5-O-phosphono-beta-D-ribofuranosylamine 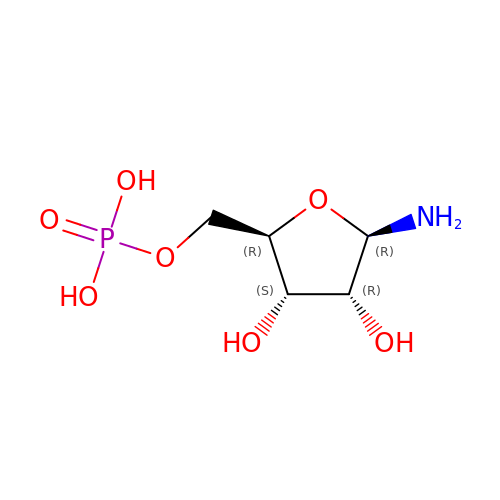| C5 H12 N O7 P | SKCBPEVYGOQGJN-TXICZTDVSA-N>MSEKNVSIVVAASVLSSGIGINGQLPWSISEDLKFFSKITNNKCDSNKKNALIMGRKTWDSIGRRPLKNRIIVVISSSLPQDEADPNVVVFRNLEDSIENLMNDDSIENIFVCGGESIYRDALKDNFVDRIYLTRVALEDIEFDTYFPEIPETFLPVYMSQTFCTKNISYDFMIFEKQEKKTLQNCDPARGQLKSIDDTVDLLGEIFGIRKMGNRHKFPKEEIYNTPSIRFGREHYEFQYLDLLSRVLENGAYRENRTGISTYSIFGQMMRFDMRESFPLLTTKKVAIRSIFEELIWFIKGDTNGNHLIEKKVYIWSGNGSKEYLERIGLGHREENDLGPIYGFQWRHYNGEYKTMHDDYTGVGVDQLAKLIETLKNNPKDRRHILTAWNPSALSQMALPPCHVLSQYYVTNDNCLSCNLYQRSCDLGLGSPFNIASYAILTMMLAQVCGYEPGELAIFIGDAHIYENHLTQLK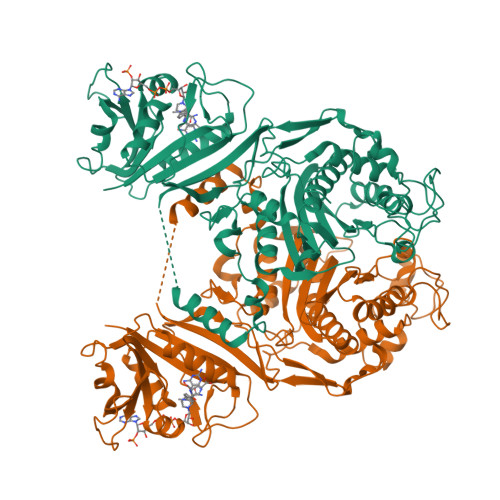EQLSRTPRPFPQLKFKRKVENIEDFKWEDIELIGYYPYPTIKMDMAV[2x]>RSPWARWFPKTLPCDVTLDVSKNHVIVDCTDKHLTEIPGGIPTNTTNLTLTINHIPDISPASFHRLVHLVEIDFRCNCVPIRLGSKSNMCPRRLQIKPRSFSGLTYLKSLYLDGNQLLEIPQGLPPSLQLLSLEANNIFSIRKEQLTELANIEILYLGQNCYYRNPCYVSYSIEKDAFLNLTKLKVLSLKDNNVTTVPTVLPSTLTELYLYNNMIAEIQEDDFNNLNQLQILDLSGNCPRCYNAPFPCTPCKNNSPLQIPVNAFDALTELKVLRLHSNSLQHVPPRWFKNINNLQELDLSQNFLAKEIGDAKFLHFLPNLIQLDLSFNFELQVYRASMNLSQAFSSLKSLKILRIRGYVFKELKSFQLSPLHNLQNLEVLDLGTNFIKIANLSMFKQFKRLKVIDLSVNKISPSGDSSEVGFCSNARTSVESYEPQVLEQLYYFRYDKYARSCRFKNKEASFTSVQESCYKYGQTLDLSKNSIFFIKSSDFQHLSFLKCLNLSGNLISQTLNGSEFQPLAELRYLDFSNNRLDLLHSTAFEELRKLEVLDISSNSHYFQSEGITHMLNFTKNLKVLQKLMMNDNDISSSTSRTMESESLRTLEFRGNHLDVLWRDGDNRYLQLFKNLLKLEELDISKNSLSFLPSGVFDGMPPNLKNLSLAKNGLKSFIWEKLRYLKNLETLDLSHNQLTTVPERLSNCSRSLKNLILKNNQIRSLTKYFLQDAFQLRYLDLSSNKIQMIQKTSFPENVLNNLKMLLLHHNRFLCTCDAVWFVWWVQHTEVTIPYLATDVTCVGPGAHK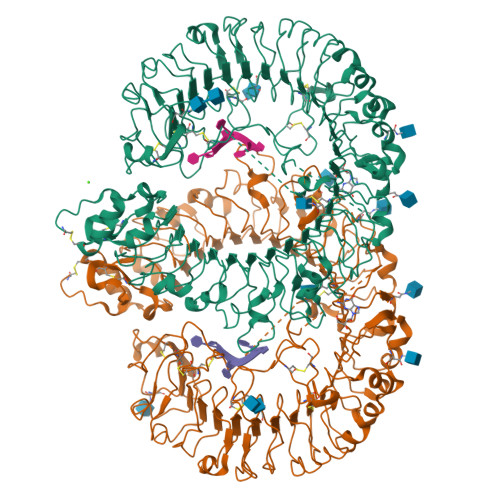GQSVISLDLYTCELDLTN[4x]> MGSSHHHHHHSSGENLYFQGQRLLGQKARMVKMYMACRNDIHRYDATFIAIYKSLIPAEEELEKQRQLMAHLENLVAKEWPHAKLYLYGSCANSFGFPKSDIDVCLAIEGDDINKSEMLLKLAEILESDNLQNVQALTRARVPIVKLMDPVTGISCAICINNVLAVVNTKLLRDYAQIDVRLRQLAFIVKHWAKSRRVNETYQGTLSSYAYVLMCIHFLQQRRPPILPCLQEMEPTYSVRVDNIRCTYFDNVDRLRNFGSNNR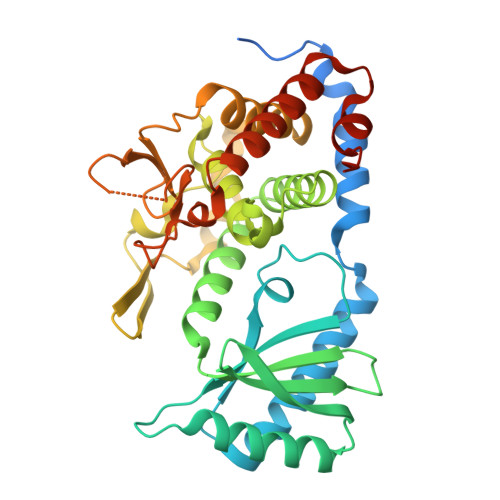ETIAELVWGFFNYWAYAHDYAYNVVSVRTGSILGKREKDWTRRVGNDRHLICIEDPFETSHDLGRVVDKFSIRVLREEFERAARIMHQDPNPCAKLLEPYIPEDNNGQGHN>GAAAGGGGAGUAGCGUCGGGAAACCGAAACAAAGUCGUCAAUUCGUGAGG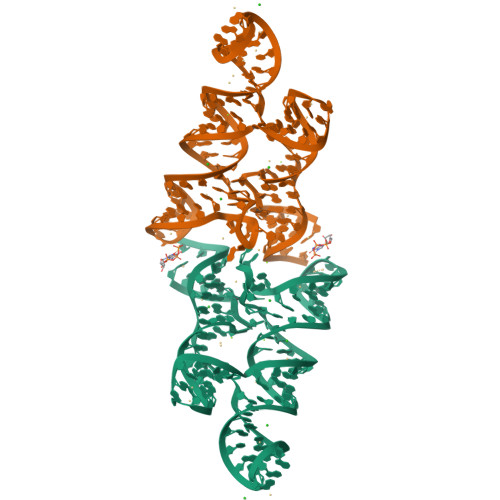AAACUCACCGGCUUUGUUGACAUACGAAAGUAUGUUUAGCAAGACCUUUCC[2x]> MPFVNKQFNYKDPVNGVDIAYIKIPNAGQMQPVKAFKIHNKIWVIPERDTFTNPEEGDLNPPPEAKQVPVSYYDSTYLSTDNEKDNYLKGVTKLFERIYSTDLGRMLLTSIVRGIPFWGGSTIDTELKVIDTNCINVIQPDGSYRSEELNLVIIGPSADIIQFECKSFGHEVLNLTRNGYGSTQYIRFSPDFTFGFEESLEVDTNPLLGAGKFATDPAVTLAHQLIHAGHRLYGIAINPNRVFKVNTNAYYEMSGLEVSFEELRTFGGHDAKFIDSLQENEFRLYYYNKFKDIASTLNKAKSIVGTTASLQYMKNVFKEKYLLSEDTSGKFSVDKLKFDKLYKMLTEIYTEDNFVKFFKVLNAKTFLNFDKAVFKINIVPKVNYTIYDGFNLRNTNLAANFNGQNTEINNMNFTKLKNFTGLFEFYKLLCVRGIITSKTKSLDKGYNKALNDLCIKVNNWDLFFSPSEDNFTNDLNKGEEITSDTNIEAAEENISLDLIQQYYLTFNFDNEPENISIENLSSDIIGQLELMPNIERFPNGKKYELDKYTMFHYLRAQEFEHGKSRIALTNSVNEALLNPSRVYTFFSSDYVKKVNKATEAAMFLGWVEQLVYDFTDETSEVSTTDKIADITIIIPYIGPALNIGNMLYKDDFVGALIFSGAVILLEFIPEIAIPVLGTFALVSYIANKVLTVQTIDNALSKRNEKWDEVYKYIVTNWLAKVNTQIDLIRKKMKEALENQAEATKAIINYQYNQYTEEEKNNINFNIDDLSSKLNESINKAMININKFLNQCSVSYLMNSMIPYGVKRLEDFDASLKDALLKYIYDNRGTLIGQVDRLKDKVNNTLSTDIPFQLSKYVDNQRLLSTFTEYIKNIINTSILNLRYESNHLIDLSRYASKINIGSKVNFDPIDKNQIQLFNLESSKIEVILKNAIVYN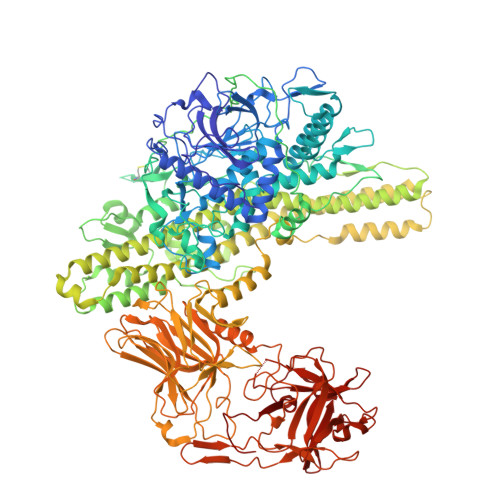SMYENFSTSFWIRIPKYFNSISLNNEYTIINCMENNSGWKVSLNYGEIIWTLQDTQEIKQRVVFKYSQMINISDYINRWIFVTITNNRLNNSKIYINGRLIDQKPISNLGNIHASNNIMFKLDGCRDTHRYIWIKYFNLFDKELNEKEIKDLYDNQSNSGILKDFWGDYLQYDKPYYMLNLYDPNKYVDVNNVGIRGYMYLKGPRGSVMTTNIYLNSSLYRGTKFIIKKYASGNKDNIVRNNDRVYINVVVKNKEYRLATNASQAGVEKILSALEIPDVGNLSQVVVMKSKNDQGITNKCKMNLQDNNGNDIGFIGFHQFNNIAKLVASNWYNRQIERSSRTLGCSWEFIPVDDGWGERPL>[2x]YYKEIAHAL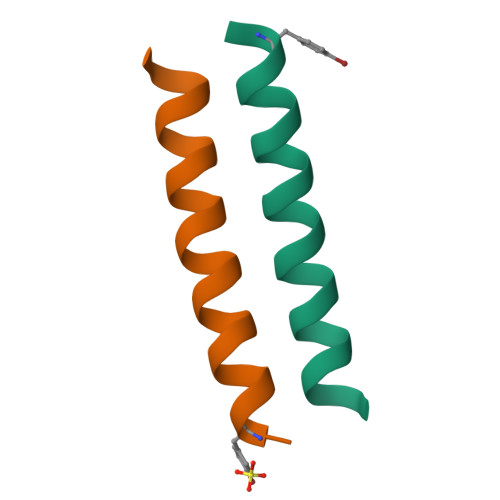FSALFALSELYIAVRYX>MNEMFSQGGKGSTGILTNKQAVARHFGVKQSEVVYFSVGVDLGGYKVIYDKETQRAYSLPVGIASGTTAVSLSTAAVLVHSAGSVDLGSLAVSREEYVTLPGSFDSGSTLNVKNELLTYTDGKYRWDGILPKTVAPGSTPASTGGVGLGAWISVGDASLRTQLANGDGSLIGIHPQGTLNNVLTVRTPEQYNAVGDGIADDTSKLKEMLSDINNVPETLPDAAAVNSYMEQVAVKIDLTKLYRFTETLYIPPGVSIEIPTSNFFTRECKQGLFYDPVDKNTAAISLMVYRKQPDGSYKLNKDVDYYPTGLDIDNGDAITCARKIDINNLNLITAPGVKVGVKWIGGAGCTTKGLSIGENTGSDITTARLPRVGLLQSASWGSIHENLRILYKTQGAVFIDSNGGAAVNNAYISRLGNTNGELEQAVYKPAGFTEVGDVAVTQFAGSEVKFNSPIIEQASFDFVHAGRDTDSYGLFMVDKPHIESSGGKKKHSFYLINTSSNVTLSGVGLSGQDPDLDSMYFLKNCPETARNVVRGQMPISGVKLVRGTGNYPTLVLDCTNMGSQFQFGEVGDIFYIKDVVGVKADTLYIDPVNGNNYNWGTNGTKPIRELTNIAKICQLFRCKSVYLNAGESVITSNTELPMVVFEGPGSLKANSGSSFLIKAGGTLSLIGLSGISTDGGHMFRVSTVEKVNIHTNCSVNAGAAYVVLSEVQGNIEYRQLFYSVNCSKYIGATAGQTIAGIMVKTATRPTGIDAAPVDGNVSLTYKIIESHHHHHH[3x]

In contrast, CBA120 contained multiple genes for putative TSPs (TSP1-TSP4), genes that are more commonly associated with Podoviridae rather than Myoviridae. Analytical gel filtration of purified TSP1 revealed a single homogeneous peak at ∼252 kDa based on regression analysis of gel filtration standards (data not shown), suggesting that similar to all other tailspike proteins with known structures, TSP1 forms a trimer in solution (predicted 82 kDa monomer, 246 kDa trimer). The TSP1 trimer assumes an elongated rod-like shape of approximately 170 Å in length and 75 Å in diameter at the widest region.

The crystal's asymmetric unit contains the biological homotrimer. The N-terminal domain (amino acid residues 12–155) that putatively attaches to the virion forms the spherical head of the trimeric assembly. In addition to electrostatic and hydrophobic interactions, oligomerization of the three head binding domains is enhanced by the coordination to the Zn2+. The C-terminal domain (amino acid residues 166–769) forms a bent 3-stranded right-handed parallel β helix. A short α-helix (amino acid residues 155–165) forms a “neck” that connects the head binding and receptor binding domains. The receptor binding domain may be further divided into two β-helical subdomains D3 (residue 166–562) and D4 (residues 624–769), intervened by a non β-helical region (residues 563–623). The inserted region introduces a 30° bend between the D3 and D4 β-helix axes. This bending produces a 13 by 16 Å channel along the trimer axis with openings to bulk solvent between each of the trimer subunits. Instead, a cluster of amino acid residues located in a groove at the interface between subunits is suggestive of catalytic machinery. This cluster includes a pair of adjacent glutamic acids that share a proton, located on the same subunits of TSP1, Glu456 and Glu483.> MATGKTSSAANLFTGSTRFDLSSADSPPSKLSLSSDQLNHCHQALGVFRGKIQNPDSIAHEFTGLQANRMWPSELLLNSTVAMNSV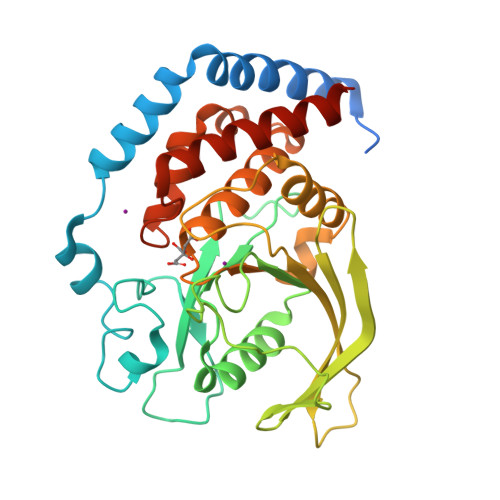NVEKNRYSDVVPFDKNRIVLNPCKDSSAKGYVNASLIKTSESESISQFIATQGPLPHTMEDFWEMVIQQHCPIIVMLTRLVDNNRTVKCGDYFQDEDGPREFGNISLTTKWIKTTDTSLMLRNLEVNYKETEDQPMSVLHIQYPEWPDHGVPKDTVAVREILKRLYQVPPSLGPIIVHCSAGIGRTGTYCAIHNTIQRILAGDMSALDLAKTVALFRKQRIGMVQTMDQYFFCYNAIVDELEDLTAGTNAGTSS> MNQPSSLAADLRGAWHAQAQSHPLITLGLAASAAGVVLLLVAGIVNALTGENRVHVGYAVLGGAAGFAATALGALMALGLRAISARTQDAMLGFAAGMMLAASAFSLILPGLDAAGTIVGPGPAAAAVVALGLGLGVLLMLGLDYFTPHEHERTGHQGPEAARVNRVWLFVLTIIL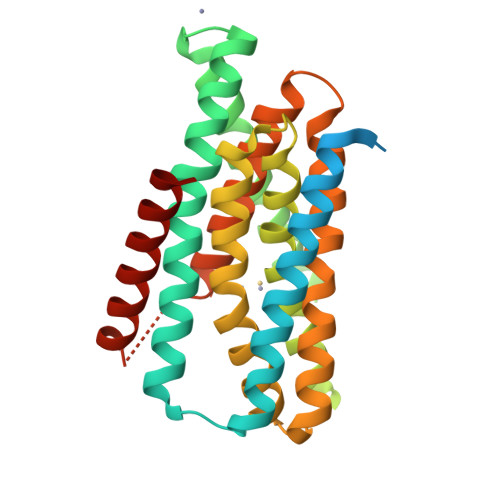HNLPEGMAIGVSFATGDLRIGLPLTSAIAIQDVPEGLAVALALRAVGLPIGRAVLVAVASGLMEPLGALVGVGISSGFALAYPISMGLAAGAMIFVVSHEVIPETHRNGHETTATVGLMAGFALMMFLDTALG In non-spherical bacteria, the actin homologue MreB is essential for shape maintenance as depletion of MreB through genetic knockouts or MreB-targeted drug treatment results in misshapen cells that eventually lyse. The MreB fibres are attached to the cell membrane via a hydrophobic loop in Thermotoga maritima as well as Gram+ bacteria and via an additional N-terminal amphipathic helix in Gram− bacteria. Here, we demonstrate that MreB from Caulobacter crescentus forms pairs of antiparallel protofilaments as revealed by crystal structures, an architecture unprecedented among actin-like proteins. The crystal structure of Caulobacter MreB (ΔCcMreBdh) reveals the typical actin fold, containing two domains on either side of a nucleotide binding cleft (Kabsch and Holmes, 1995).

In contrast, the crystals of Caulobacter MreB contain doublets that, remarkably, crystallised in an antiparallel arrangement. Upon polymerisation, domain IB shows a rotation of 21.7° towards the nucleotide binding cleft as analysed by Dyndom (Hayward and Lee, 2002). This domain closure is accompanied by a twist between domains IA and IIA, as can be appreciated from the top view in Figure 6—figure supplement 2D and from the schematic in Figure 6C. The interdomain cleft narrows due to the movement of domain I towards domain II that is accompanied by a rotation of domain I resulting in flattening of the interfilament interface. The relatively small conformational change upon polymerisation has a dramatic effect on the chemistry of the active site. In the AMPPNP protofilament conformation, the active site residues E140 and T167 coordinate a water molecule that is in line for the hydrophilic attack on the gamma phosphate. The catalytic site residues E140 and T167 coordinate the attacking water to be in line with the gamma phosphate in filamentous MreB (pink). In both proteins, the active site geometry in the filament conformation favours nucleotide hydrolysis, which is driven by a catalytic glutamate (E140 in CcMreB and E148 in ParM) that positions the catalytic water in line with the gamma phosphate. From the ΔCcMreBdh co-crystal structures with ADP and AMPPNP, it is clear that the active site could well accommodate a guanidine instead of an adenine as the major contacts are with the ribose and phosphate moieties of the nucleotide, a feature, again, shared with ParM.

>[2x]MISNDIAIDLGTANTLIYQKGKGIVLNEPSVVALRNVGGRKVVHAVGIEAKQMLGRTPGHMEAIRPMRDGVIADFEVAEEMIKYFIRKVHNRKGSGNPKVIVCVPSGATAVERRAINDSCLNAGARRVGLIDEPMAAAIGAGLPIHEPTGSMVVDIGGGTTEVAVLSLSGIVYSRSVRVGGDKMDEAIISYMRRHHNLLIGETTAERIKKEIGTARAPADGEGLSIDVKGRDLMQGVPREVRISEKQAADALAEPVGQIVEAVKVALEATPPELASDIADKGIMLTGGGALLRGLDAEIRDHTGLPVTVADDPLSCVALGCGKVLEHPKWMKGVLESTLAGSHHHHHH> MAVPETRPNHTIYINNLNEKIKKDELKKSLHAIFSRFGQILDILVSRSLKMRGQA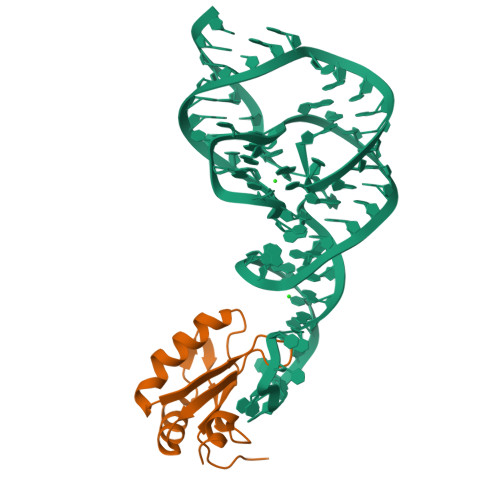FVIFKEVSSATNALRSMQGFPFYDKPMRIQYAKTDSDIIAKMKGT>MAGWNAYIDNLMADGTCQDAAIVGYKDSPSVWAAVPGKTFVNITPAEVGVLVGKDRSSFYVNGLTLGGQKCSVIRDSLLQDGEFSMDLRTKSTGGAPTFNVTVTKTDKTLVLLTGKEGVHGGLINKKCYEMASHLRRSQY[2x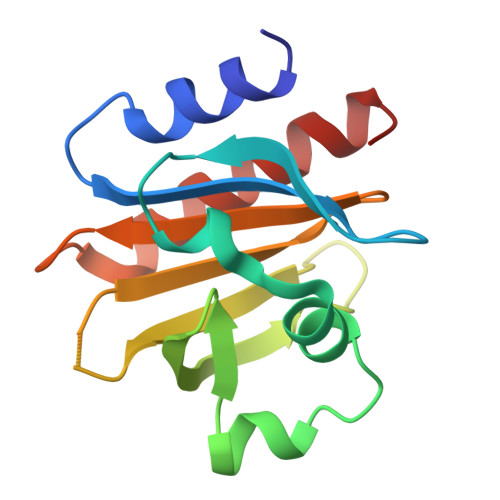]> GPSRQGWQAFKNDATEIIPELGEYPEPPPELENNKTMNRAENGGRPPHHPFETKDVSEYSCRELHFTRYVTDGPCRSAKPVTELVCSGQCGPARLLPNAIGRGKWW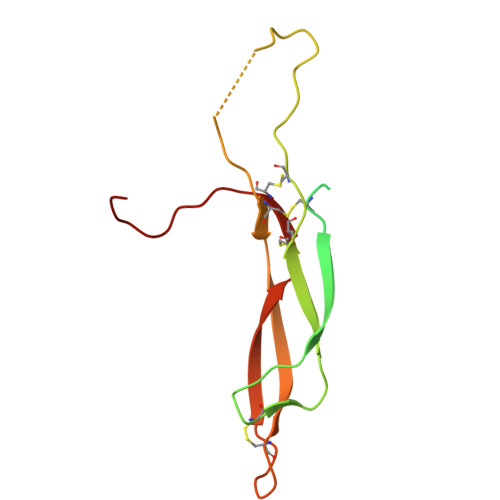RPSGPDFRCIPDRYRAQRVQLLCPGGEAPRARKVRLVASCKCKRLTRFHNQS>MNSKCHCVILNDGNFIPVLGFGTALPLECPKSKAKELTKIAIDAGFHHFDSASVYNTEDHVGEAIRSKIADGTVRREDIFYTSKVWCTSLHPELVRASLERSLQKLQFDYVDLYLIHYPMALKPGEENFPVDEHGKLIFDRVDLCATWEAMEKCKDAGLTKSIGVSNFNYRQLEMILNKPGLKYKPVCNQVECHPYLNQMKLLDFCKSKDIVLVAYGVLGTQRYGGWVDQNSPVLLDEPVLGSMAKKYNRTPALIALRYQLQRGIVVLNTSLKEERIKENMQVFEFQLSSEDMKVLDGLNRNMRYIPAAIFKGHPNW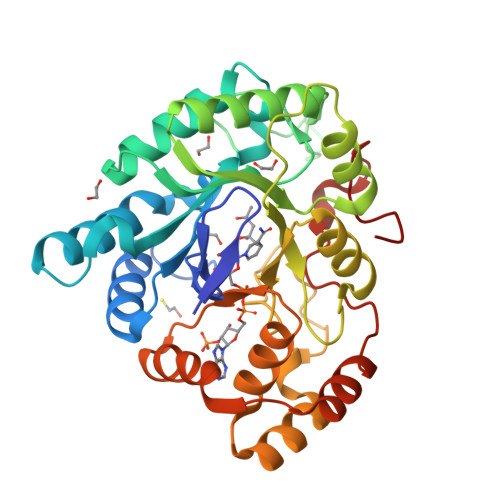PFLDEY[2x]> PISPIETVPVKLKPGMDGPKVKQWPLTEEKIKALVEICTEMEKEGKISKIGPENPYNTPVFAIKKKDSTKWRKLVDFRELNKRTQDFWEVQLGIPHPAGLKKKKSVTVLDVGDAYFSVPLDEDFRKYTAFTIPSINNETPGIR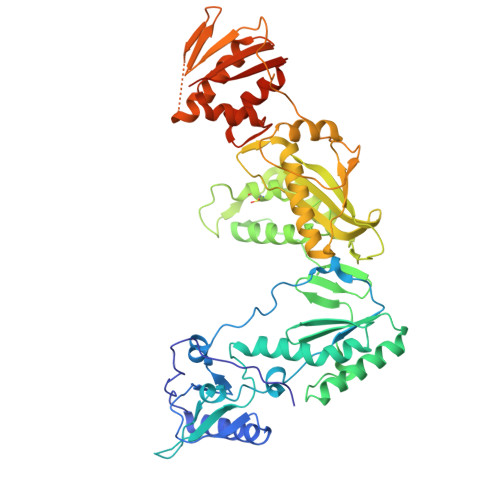YQYNVLPQGWKGSPAIFQSSMTKILEPFRKQNPDIVIYQYVDDLYVGSDLEIGQHRTKIEELRQHLLRWGLTTPDKKHQKEPPFLWMGYELHPDKWTVQPIVLPEKDSWTVNDIQKLVGKLNWASQIYPGIKVRQLCKLLRGTKALTEVIPLTEEAELELAENREILKEPVHGVYYDPSKDLIAEIQKQGQGQWTYQIYQEPFKNLKTGKYARMRGAHTNDVKQLTEAVQKITTESIVIWGKTPKFKLPIQKETWETWWTEYWQATWIPEWEFVNTPPLVKLWYQLEKEPIVGAETFYVDGAANRETKLGKAGYVTNRGRQKVVTLTDTTNQKTELQAIYLALQDSGLEVNIVTDSQYALGIIQAQPDQSESELVNQIIEQLIKKEKVYLAWVPAHKGIGGNEQVDKLVSAGIRKVL>MQPKLTIWCSEKQVDILQKLGEEFKAKYGVEVEVQYVNFQDIKSKFLTAAPEGQGADIIVGAHDWVGELAVNGLIEPIPNFSDLKNFYETALNAFSYGGKLYGIPYAMEAIALIYNKDYVPEPPKTMDELIEIAKQIDEEFGGEVRGFITSAAEFYYIAPFIFGYGGYVFKQTEKGLDVNDIGLANEGAIKGVKLLKRLVDEGILDPSDNYQIMDSMFRE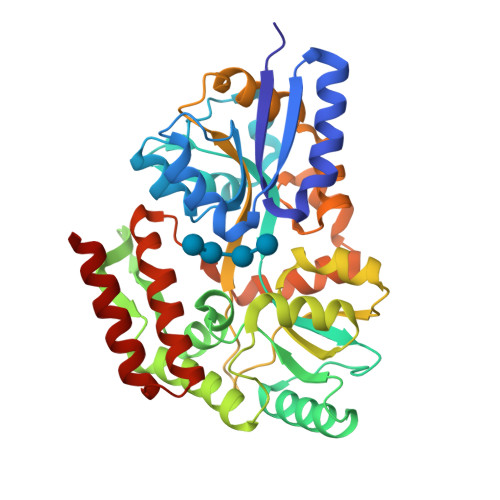GQAAMIINGPWAIKAYKDAGIDYGVAPIPDLEPGVPARPFVGVQGFMVNAKSPNKLLAIEFLTSFIAKKETMYRIYLGDPRLPSRKDVLELVKDNPDVVGFTLSAANGIPMPNVPQMAAVWAAMNDALNLVVNGKATVEEALKNAVERIKAQIQS[2x]> DEYEIIETIGNGAYGVVSSARRRLTGQQVAIKKIPNAFDVVTNAKRTLRELKILKHFKHDNIIAIKDILRPTVPYGEFKSVYVVLDLMESDLHQIIHSSQPLTLEHVRYFLYQLLRGLKYMHSAQVIHRDLKPSNLLVNENCELKIGDFGMARGLCTSPAEHQYFMTEYVATRWYRAPELMLSLHEYTQAIDLWSVGCIFGEMLARRQLFPGKNYVHQLQLIMMVLGTPSPAVIQAVGAERVRAYIQSLPPRQPVPWETVYPGADRQALSLLGRMLRFEPSARISAAAALRHPFLAKYHDPDDEPDCAPPFDFAFDREALTRERIKEAIVAEIEDFHARRE

The ERK5 protein, which is encoded by the MAPK7 gene, comprises an N-terminal kinase domain and a large C-terminal domain containing transcriptional transactivating functionality and nuclear localization and export sequences (NLS/NES). ERK5 is the effector kinase of a canonical kinase module comprising MEK (MAPK/ERK kinase) 5, MEKK (MEK kinase) 2/3 and ERK5 itself.

Compounds 4–6 are close analogues of one another. Compounds 4, 5 and 6 bind at a different binding site to compounds 1, 2 and 3. This site lies adjacent to the ATP-binding site. As observed for the complex of compound 1 with ERK5, compounds 2–5 bind to a ‘DFG-in’ conformation of ERK5 in which both the hydrophobic R-spine (residues Leu106, Ile117, His180 and Phe201 in ERK5) and C-spine (Val69, Ala82, Leu144, Leu188, Leu189, Val190, Ile251 and Met255) are intact. Compared with the structures of ERK5 in complex with the hinge-binding compounds 1–3, however, the P-loop is pushed away from the αC helix towards the ATP-binding site upon allosteric inhibitor binding (compare the grey and coral P-loops). Differential flexibility in the P-loop amongst kinases has been implicated in the selectivity of certain conventional ATP-binding site-targeted kinase inhibitors, and may have implications for the selectivity of our allosteric ERK5 inhibitors (see §3.5). In contrast to the P-loop, the αC helix orientation is unchanged upon the binding of compounds 4–6. The side chain of Lys84 is displaced by binding of compounds 4–6 and reorients to form a hydrogen bond to the backbone carbonyl of Val68 from the P-loop.Vandetanib | C22 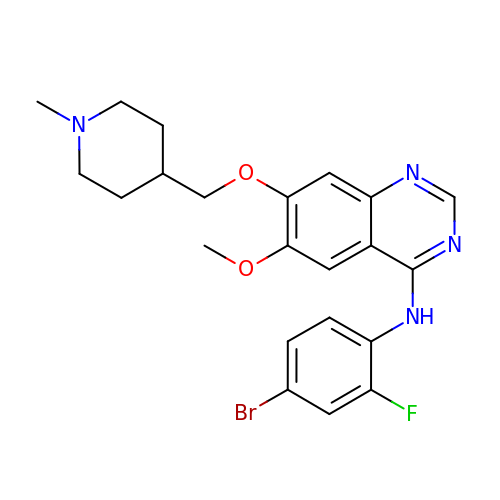H24 Br F N4 O2 | UHTHHESEBZOYNR-UHFFFAOYSA-N> MADKELKFLVVDKFSTMRRIVRNLLKELGFNNVEEAEDGVDALNKLQAGGFGFIISDWNMPNMDGLELLKTIRADSAMSALPVLMVTAEAKKENIIAAAQAGASGWVVKPFTAATLEEKLNKIFEKL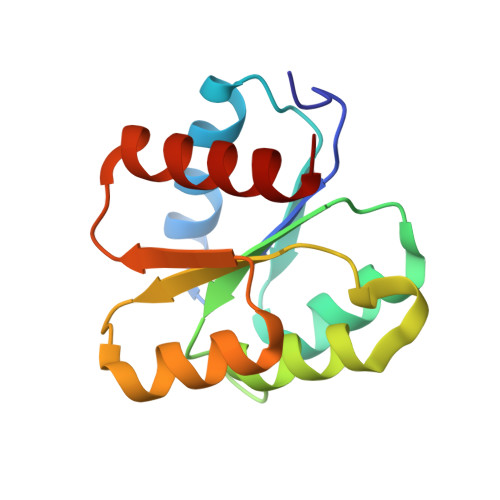GM> HWKTRAVPGAGTFGSAVAGQELPLCGVRAYYPPNAYIPAQVRDWLEFAHRPGL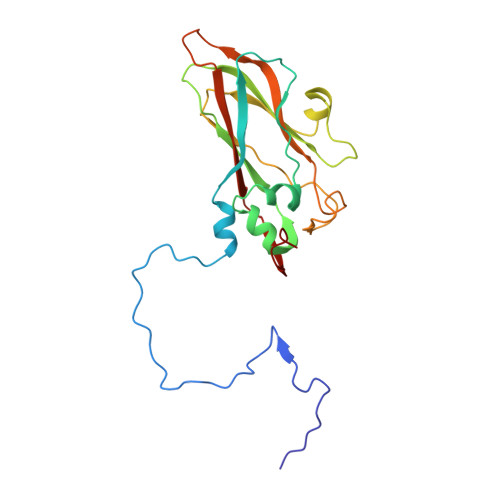MATVPWTMADEPAERLGIFPVSPSAIAGTGAPISYVISLFSQWRGELAAHLLFTGSAQHYGRLVVCYTPAAPQPPSTMQEAMRGTYTVWDVNAASTLEFTIPFISNSYWKTVDVNNPDALLSTTGYVSIWVQNPLVGPHTAPASALVQAFISAGESFNVRLMQNPALTS>[4x]MGSQFLLSVREFMQTRYYAKKTIEAYLHWITRYIHFHNKKHPSLMGDKEVEEFLTYLAVQGKVATKTQSLALNSLSFLYKEILKTPLSLEIRFQRSQLERKLPVVLTRDEIRRLLEIVDPKHQLPIKLLYGSGLRLMECMRLRVQDIDFDYGAIRIWQGKGGKNRTVTLAKELYPHLKEQIALAKRYYDRDLHQKNYGGVWLPTA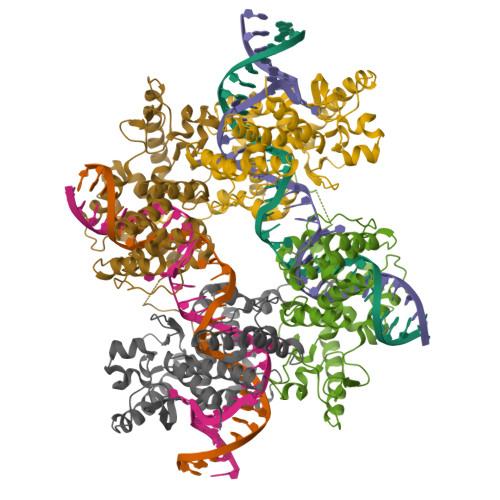LKEKYPNAPYEFRWHYLFPSFQLSLDPESDVMRRHHMNETVLQKAVRRSAQEAGIEKTVTCHTLRHSFATHLLEVGADIRTVQEQLGHTDVKTTQIYTHVLDRGASGVLSPLSRL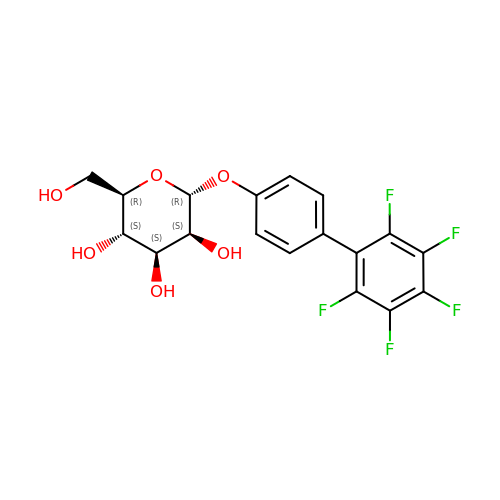(2~{R},3~{S},4~{S},5~{S},6~{R})-2-(hydroxymethyl)-6-[4-[2,3,4,5,6-pentakis(fluoranyl)phenyl]phenoxy]oxane-3,4,5-triol | C18 H15 F5 O6 | WCSHODXKNWBNJL-VYMSMKAZSA-N>[4x]MKKIYLIRHAQSEYNEKGIFQGRLDSDLTPLGFVQSRLLVKQFEREKPEVIITSPQRRAYKTALTLSDV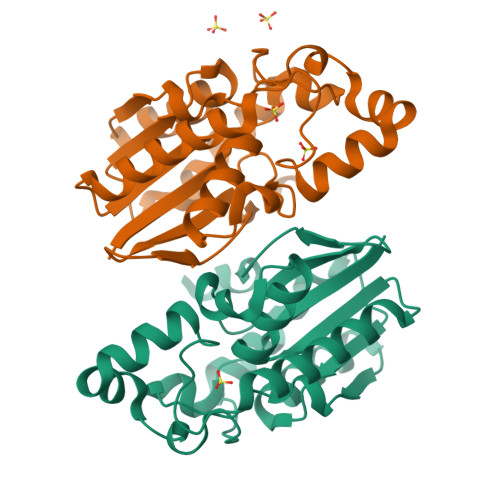LGIDLIVDERIREMSFGVLEGRHFWTMFEENKEMIINWLKDPVKYPLPTQEDIKEFEKRIKEFLEDLKSRKEKVLAVVGHGGTLHGLLCLALGIGLEKMWHIHMDNTGISLLEYDGERFYLKSLNDTCHLLVLD> MGHHHHHHMVLADLGRKITSALRSLSNATIINEEVLNAMLKEVCTALLEADVNIKLVKQLRENVKSAIDLEEMASGLNKRKMIQHA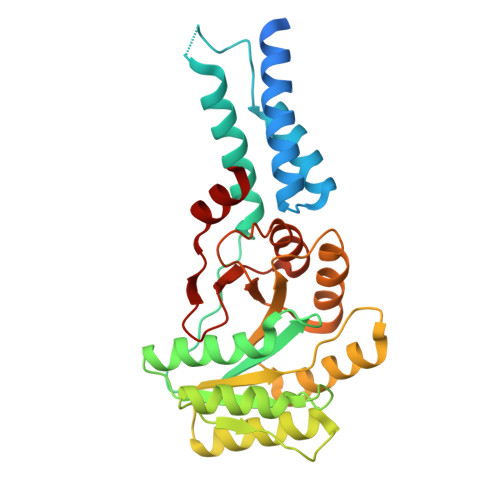VFKELVKLVDPGVKAWTPTKGKQNVIMFVGLQGSGKTTTCSKLAYYYQRKGWKTCLICADTFRAGAFDQLKQNATKARIPFYGSYTEMDPVIIASEGVEKFKNENFEIIIVDTSGRHKQEDSLFEEMLQVANAIQPDNIVYVMDASIGQACEAQAKAFKDKVDVASVIVTKLDGHAKGGGALSAVAATKSPIIFIGTGEHIDDFEPFKTQPFISKLLG>MEFIKGFTFGWDSQKGYFKTERAKESLRLMQERTASEYVIVALAALQDTAHSTEVDFQGSHMVDDDELIELIDYAKSLGLKVILKPTVNCRNGTWRAHINFFDMDIPGEPTWDEWFESYINYQKHYAKIAEKTNCEMFVVGCEMVQAERREDKWRELIAEVRKDYRGLVTYNTDKYQEDNVKFWDALDVISSSGYYPINDWDRQLDRIEAVVKQYDKPFFFVEAGCPSRSGSALLPNKWD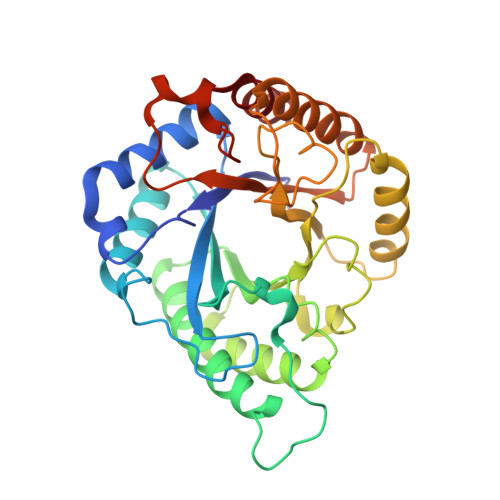LEGAINLQEQADYYQVMFEKTASRSWVGGFGLWDWQTYLYDEKDATKNDDYGVFGKPAERVIKAYYQSR[2x]> MALDLSSGFAAADAIANLQLADATLPIFEVLPVQLQFSVAADFVAGQAANNVLVIALSNGRILRIDLNKPEDIDDIDLPKKPSEVGVIRRMFLDPTASHLIICTSLGENYYLHSQSRQPRPLARLRGVVIESIAWSPALPTQSTREILIGAADGNIYEAYIETSTEFYRREDKYLKLVQKLPDGPITGLWADSLPGHKDTRRVLVATSSRLFHWVGKIGRGHDSGGGASIYDKLFEAEQPTVHALSGASAAAMSMLVVSPDAEQPSPRFREDEVPERAFAWLSSHGVYHGKLLLKGPLSELGAKVFAEAKLLPRAQLANPEGASRRQLSTEYVDAVALTQWHIVSLVAGRVVIANRLTGSIIYDQTILNPGQKAVGLCVDQQKSTFWLFTPQEIFEIVPRDEDRDIWKIMLQLQQFDAALQYAHTPAEKDAVAIASGDHLVSKGQFLEAAAVYGKSSKPFEEVALTFIDNEQPDALRKYLLTKLGTYKKSAVMQRVMIATWLIEVFMAKLNSLDDTIITGAELSETLNPNQTKEQLEAVRAEFQDFINKHKGDLDRKTVYDVIGSHGREEELLYYANAINDYNYVLSYWVQRERWTEALKVLKKQTDPEVFYRYSSVLMTHAATELVEILMRQSNLNPRNLIPAMLEYDRNYKGPLAQNQAVRYLLYVVNQLGSTDSAVHNTLVSIYASHPSK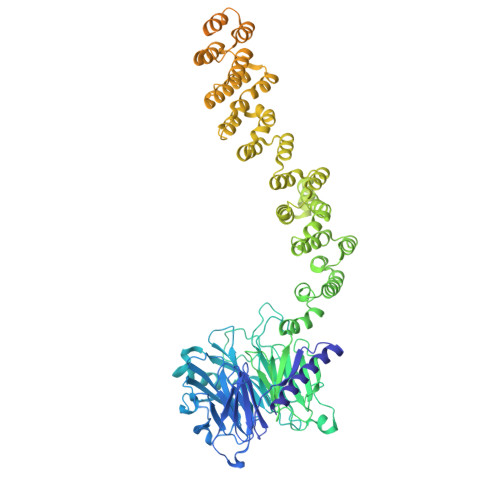DESALLEYLESQGEEPNYDPDFALRLCIQHRRVLSCAHIYTSMGQYGAAVDLALAHDEVELASIIADRPISNPQLRKKLWLKVAKKVISQQSDGIKTAIDFLRRCDLLKIEDLIPFFPDFVVIDDFKEEICAALEDYSRNIDALRREMDEASQTAANIKVDIAALDKRYAIVEPGEKCYACGLPLLSRQFFVFPCQHAFHSDCLARRVLEQAPPAKARRIKECQVQISKGLVNGEKREAMIAELDALIASACDYAIRRINEPFIKDDDDKDEWAL> GSHMKNSVSVDLPGSMKVLVSKSSNADGKYDLIATVDALELSGTSDKNNGSGVLEGVKADASKVKLTI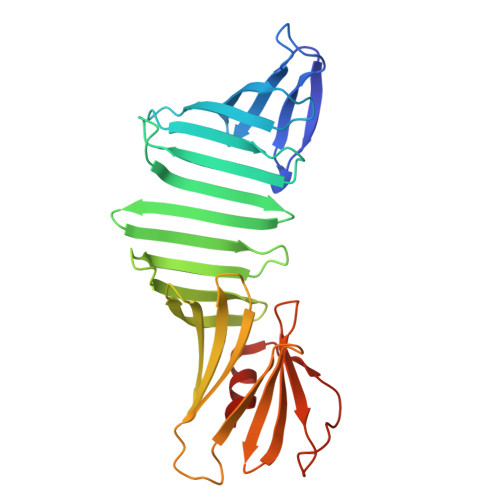SDDLGQTTLEVFKSDGSTLVSKKVTSNGSSTEEKSSNGSSEKIITRADGTRLEYTGIKSDGSGKAKEVLKGYVLEGTLTAEKTTLVVKEGTVTLSKNISKSGEVSVELNDTDSSAATKKTAAWNSGTSTLTITVNSKKTKDLVFTSSNTITVQQYDSNGTSLEGSAVEITKLDEIKNALK>MAHHHHHHMPGSELISGGWFREENDQWPGQAMSLRVEKVLYDAPTKFQHLTIFESDPKGPWGTVMALDGCIQVTDYDEFVYHEVLGHTSLCSHPKPERVLIIGGGDGGVLREVLRHGTVEHCDLVDIDGEVMEQSKQHFPQISRSLADPRATVRVGDGLAFVRQTPDNTYDVVIIDTTDPAGPASKLFGEAFYKDVLRILKPDGICCNQGESIWLDLELIEKMSRFIRETGFASVQYALMHVPTYPCGSIGTLVCSKKAGVDVTKPLRPVEDMPFAKDLKYYDSEMHKASFALPRFARHINNSE[4x]

In this study, to demonstrate the utility of virtual screening with protein dynamics, MD simulations were performed on Trypanosoma cruzi spermidine synthase to obtain an ensemble of dominant binding sites with a high probability of existence. The structure of the binding site obtained through MD simulation revealed pockets in addition to the active site that was present in the initial structure. Using the obtained binding site structures, virtual screening of 4.8 million compounds by docking simulation, in vitro assays, and X-ray analysis was conducted, successfully identifying two hit compounds.

As a result, TcSpdSyn IC50 values for two compounds were determined, with compounds 1 and 2 inhibiting TcSpdSyn at IC50 values of 82.27 and 43.41 μM, respectively. To examine the binding sites used by these two active compounds, we conducted X-ray crystallographic analyses to observe the structures of the TcSpdSyn complex with the two top-ranked compounds (compounds 1 and 2) in the hidden binding pocket, as predicted by the MD simulations. Compound 1 interacts with Glu22 and Asp77 (interaction energy values: −25.93 and −17.56 kcal/mol, respectively) through two hydrogen bonds. Therefore, these interactions would appear to be important for binding to the site. Some other interactions were also found: Trp61, Ile71, Thr244, and Tyr245 interacted with compound 1 with interaction energies of −4.45, −6.51, −4.83, and −7.36 kcal/mol, respectively. Comparing the structures of compounds 1 and 2, both are para-substituted anisoles with nitrogen-rich heterocycle para-substituents. Compound 1 interacts with Glu22 through the hydroxy group at the meta-position of anisoles, while compound 2 interacts with Glu22 via a secondary amine at para-substituent. Upon examination of the X-ray structure of TcSpdSyn with compound 1 at the binding site, the amino acid sequence overlap with the clustering structure was 72.2%. Glu22, which interacts with 1, is a feature of the sequence of the clustering structure binding site.>SNAFTGGALQVEAKEKTGQVKHKNQATHKEFSQLEKKFDARLGVYAIDTGTNQTISYRSNERFAFASTYKALAAGVLLQQNSIDSLNEVITYTKEDLVDYSPVTEKHVDTGMKLGEIAEAAVRSSDNTAGNILFNKIGGPKGYEKALRHMGDRITMSDRFETELNEAIPGDIRDTSTAKAIATNLKAFTVGNALPAEKRKILTEWMKGNATGDKLIRAGVPTDWV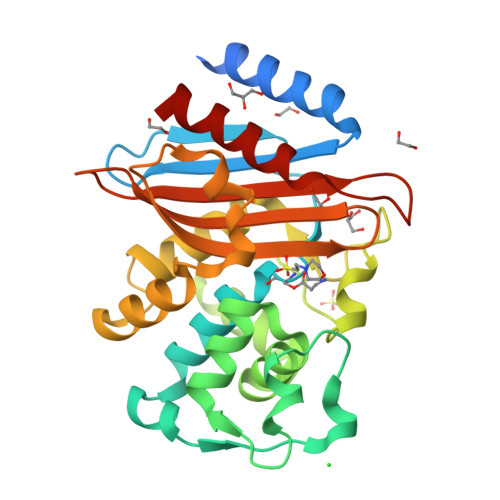VGDKSGAGSYGTRNDIAIVWPPNRTPIIIAILSSKDEKEATYDNQLIAEATEVIVKALK[2x]>SKYQVLTVGNPNSGKTTLFNGLTGAKQQVGNWAGVTVEKKTGSFVHAGDEFSLTDLPGIYALDSGNDSNSIDESIASRAVLTHPADVIINVVDATCLERSLYMTLQLRELRRPMIVVLNKMDALKRERVHLDLKQLEAFLGCPVLALSANNKEQVRRFKEKLHKLLVQGIALKQIELHYGAEFESLIHELEPMFAEQAVSARALAIRALENDRLVINGLKEAERQNVEQRQHECQVDIDLLVANVRYTYLHELCTHVRRTE[2x]

For this bacterium, Feo is the primary system that transports Fe2+ into the cytosol. FeoA and FeoC are known to be small (ca. 7–10 kDa) cytosolic proteins, while FeoB is a large (ca. 80–100 kDa) polytopic transmembrane protein that contains an N-terminal soluble G-protein-like domain termed NFeoB. The status of GTP and GDP bound to the NFeoB region is hypothesized to control the opening and closing of the FeoB pore and therefore the translocation of Fe2+ into the bacterial cytosol.

To overcome this issue, VcNFeoB was recloned into a vector encoding for N-terminal (His)6 tag fused to a cleavable SUMO moiety. Expression and purification followed the same procedures as previously described (vide supra), and the SUMO tag was cleaved prior to crystallization. Crystals of the SUMO-cleaved apo domain were generated and ultimately diffracted to 2.3 Å resolution in the P121 space group consistent with 2 molecules in the asymmetric unit (ASU). Using the 3.7 Å resolution model, we were able to solve the 2.3 Å resolution structure of the tagless protein (Rw/Rf = 0.203/0.266). The X-ray crystal structure of the apo VcNFeoB NTPase domain reveals the presence of a typical NFeoB fold. Distinctly present are the two common NFeoB subdomains: the globular G-protein subdomain that is responsible for binding and hydrolyzing nucleotides (blue) and the hammer-shaped guanine-dissociation inhibitor (GDI) subdomain that regulates nucleotide dissociation and connects directly to the FeoB transmembrane region (red). Within the G-protein domain, two switch regions (known as Switch I and Switch II) that regulate nucleotide hydrolysis and communicate nucleotide status to the GDI domain are present, albeit Switch I is mostly disordered, while Switch II is mostly ordered in the apo form. Surprisingly, a comparison of the VcNFeoB NTPase domain to other structurally characterized NFeoB domains displays strong structural conservation in both subdomains (Cα RMSD <1 Å on average) even though the NFeoB is not a strict GTPase. These observations indicate that gross structural changes in the NFeoB region do not account for the observed nucleotide promiscuity of V. cholerae FeoB per se.>NLKPVDAMQCFDCHTQIEDMHTVGKHATVNCVHCHDATEHVETASSRRMGERPVTRMDLEACATCHTAQFNSFVEVRHESHPRLEKATPTSRSPMFDKLIAGHGFAFEHAEPRSHAFMLVDHFVVDRAYGGRFQFKNWQKVTDGMGAVRGAWTVLTDADPESSDQRRFLSQTATAANPVCLNCKTQDHILDWAYMGDEHEAAKWSRTSEVVEFARDLNHPLNCFMCHDPHSAGPRVVRDGLINAVVDRGLGTYPHDPVKSEQQGMTKVTFQRGREDFRAIGLLDTADSNVMCAQCHVEYNCNPGYQLSDGSRVGMDDRRANHFFWANVFDYKEAAQEIDFFDFRHATTGAALPKLQHPEAETFWGSVHERNGVACADCHMPKVQLENGKVYTSHSQRTPRDMMGQACLNCHAEWTEDQALYAIDYIKNYTHGKIVKSEYWLAKMIDLFPVAKRAGVSEDVLNQARELHYDAHLYWEWWTAENSVGFHNPDQARESLMTSISKSKEAVSLLNDAIDAQVA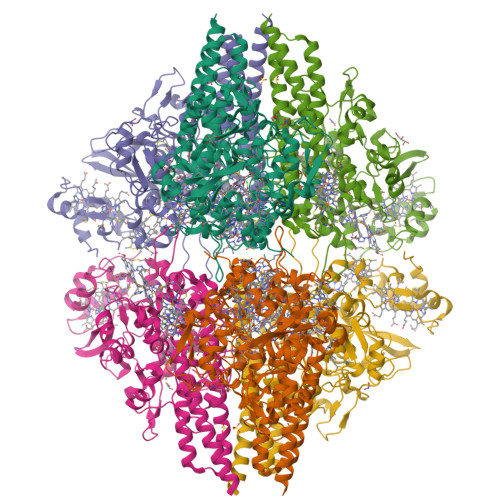V[2x]> MSGSHHHHHHSSGENLYFQGELFRGVLHISSNILDCANDNWWCSMLDLDTSDWEPLTHSNRLMAIYLSNVASRLDFTGGP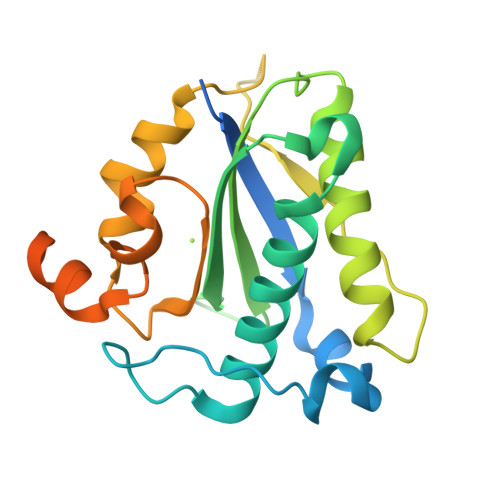LAGCLYFFQVECNKFEEGYHIHVVIGGPGLNARNLTVCVEGLFNNVLYHLVNESVKLKFLPGMTTKGKYFRDGEQFIENYLMKKIPLNVVWCVTNIDGYIDTCISASFRRGACHAKKPRISANTDTVNNEGGESSCGGGDVVPFAGKG>[2x]MAKKTSSKGKLPPGPFPLPIIGNLFQLELKNIPKSFTRLAQRFGPVFTLYVGSQRMVVMHGYKAVKEALLDYKDEFSGRGDLPAFHAHRDRGIIFNNGPTWKDIRRFSLTTLRNYGMGKQGNESRIQREAHFLLE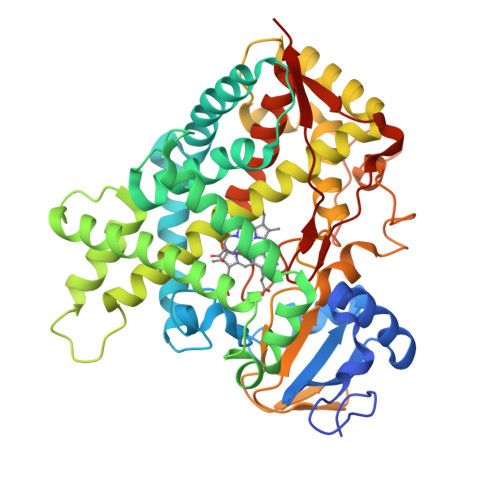ALRKTQGQPFDPTFLIGCAPCNVIADILFRKHFDYNDEKFLRLMYLFNENFHLLSTPWLQLYNNFPSFLHYLPGSHRKVIKNVAEVKEYVSERVKEHHQSLDPNCPRDLTDCLLVEMEKEKHSAERLYTMDGITVTVADLFFAGTETTSTTLRYGLLILMKYPEIEEKLHEEIDRVIGPSRIPAIKDRQEMPYMDAVVHEIQRFITLVPSNLPHEATRDTIFRGYLIPKGTVVVPTLDSVLYDNQEFPDPEKFKPEHFLNENGKFKYSDYFKPFSTGKRVCAGEGLARMELFLLLCAILQHFNLKPLVDPKDIDLSPIHIGFGCIPPRYKLCVIPRSHHHH> AYTTFSQTKNDQLKEPMFFGQPVNVARYDQQKYDIFEKLIEKQLSFFW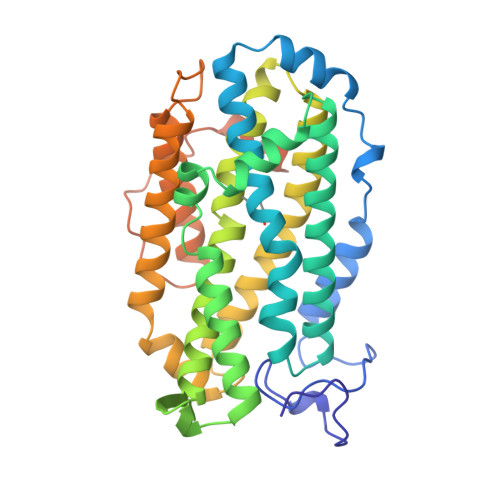RPEEVDVSRDRIDYQALPEHEKHIFISNLKYQTLLDSIQGRSPNVALLPLISIPELETWVETWAFSETIHSRSFTHIIRNIVNDPSVVFDDIVTNEQIQKRAEGISSYYDELIEMTSYWHLLGEGTHTVNGKTVTVSLRELKKKLYLCLMSVNALEAIRYYVSFACSFAFAERELMEGNAKIIRLIARDAALHLTGTQHMLNLLRSGADDPEMAEIAEECKQECYDLFVQAAQQEKDWADYLFRDGSMIGLNKDILCQYVEYITNIRMQAVGLDLPFQTRSNPIPWINTWLVSDNVQVAPQEVEVSSYLVGQIDSEVDTDDLSNFQL The adjacent fibrinogen (Fg)- and fibronectin (Fn)-binding sites on Fn-binding protein A (FnBPA), a cell surface protein from Staphylococcus aureus, are implicated in the initiation and persistence of infection. The N-terminal region of FnBPA contains three subdomains N1–N3; N2N3 binds fibrinogen (Fg) and elastin. Here, we solved the structure of the N2N3 domains containing the Fg-binding site of FnBPA in the apo form and in complex with a Fg peptide. The Fg binding mechanism is similar to that of homologous bacterial proteins but without the requirement for “latch” strand residues.

However, only rFnBPA(189–505) produced diffracting crystals. The structure of rFnBPA(189–505) comprises two distinct β-strand-dominated domains, N2 and N3, connected by an eight-residue linker. The N-terminal N2 domain (residues 195–335) consists of nine β-strands arranged in a sandwich of four- and five-strand β-sheets. The N3 domain (residues 344–503) has a similar structure comprising two β-sheets, each formed by five β-strands. However, unlike N2, the two β-sheets within the N3 domain are linked by a short helix. The structures of both domains resemble a distorted β-barrel rather than a typical β-sandwich. The N2 domain adopts the DE variant of a C-type IgG fold (DEv-IgG) identified in other proteins including ClfA. The asymmetric unit comprises a single copy of rFnBPA(189–505); no density was observed for the N- and C-terminal residues (residues 189–194 and 504–505, respectively). In the apo-form, the G′ strand aligns anti-parallel to the neighboring F′ strand.

> GPAMAKVETGTDVTSKVTVEIGSIEGHNNTNKVEPHAGQRAVLKYKLKFENGLHQGDYFDFTLSNNVNTHGVSTARKVPEIKNGSVVMATGEVLEGGKIRYTFTNDIEDKVDVTAELEINLFIDPKTVQTNGNQTITSTLNEEQTSKELDVKYKDGIGNYYANLNGSIETFNKANNRFSHVAFIKPNNGKTTSVTVTGTLMKGSNQNGNQPKVRIFEYLGNNEDIAKSVYANTTDTSKFKEVTSNMSGNLNLQNNGSYSLNIENLDKTYVVHYDGEYLNGTDEVDFRTQMVGHPEQLYKYYYDRGYTLTWDNGLVLYSNKA5-chloro-2-methoxy-N-(2-methyl[1,2,4]triazolo[1,5-a]pyridin-8-yl)benzene-1-sulfonamide | C14 H13 Cl N4 O3 S | 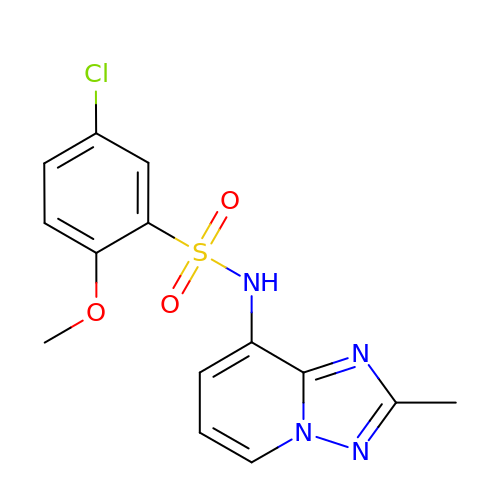HLRMNXITZQAUIH-UHFFFAOYSA-N(3~{S})-3-[2,6-bis(fluoranyl)phenyl]-~{N}-[(2-oxidanylidene-1,3-dihydrobenzimidazol-5-yl)methyl]butanamide | C18 H17 F2 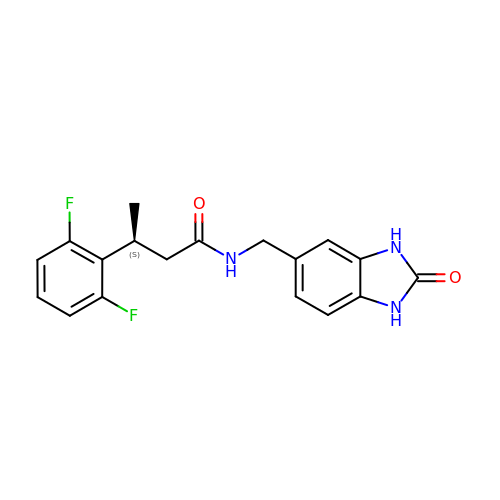N3 O2 | VDLFVZUKOKPJRH-JTQLQIEISA-N> MSEKNREHSHRHNHEHKYRKQVINRLARIEGHVRAIKEMAAEGRDCPDILLQIAAVRKALDSTAKVIFADHMESCLVDAVH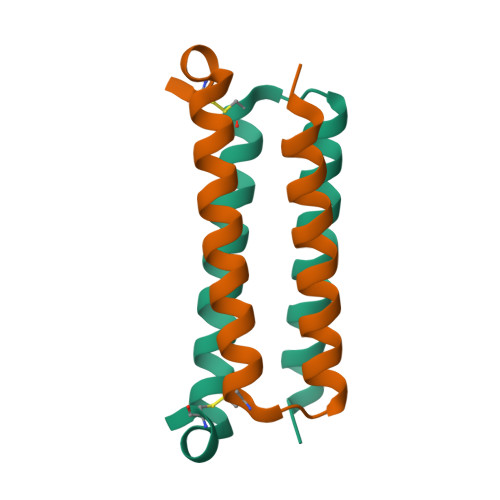QGNEDQVLNDLKKLHHHHHH>MTQQITLIKDKILSDNYFTLHNITYDLTRKDGEVIRHKREVYDRGNGATILLYNTKKKTVVLIRQFRVATWVNGNESGQLIESCAGLLDNDEPEVCIRKEAIEETGYEVGEVRKLFELYMSPGGVTELIHFFIAEYSDNQRANAGGGVEDEDIEVLELPFS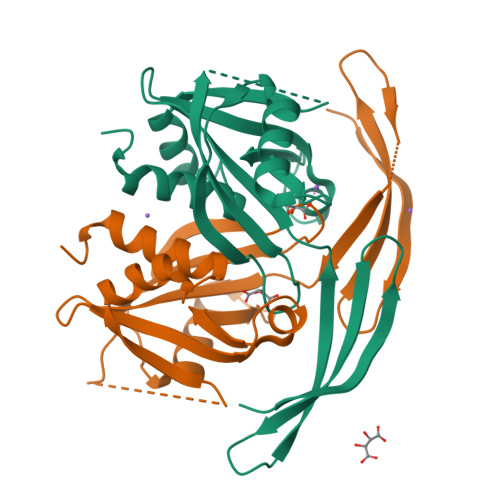QALEMIKTGEIRDGKTVLLLNYLQTSHLMD[5x]> GSMQANQWQSVQNRTFTKWFNTKLSSRDLPSVFDLRKDLSDGILLIQLLEIIGDENLGRYNRNPRMRVHRLENVNKALEYIKSKGMPLTNIGPADIVDGNLKLILGLIWTLILRFTIADINEEGLTAKEGLLLWCQRKTANYHPEVDVQDFTRSWTNGLAFCALIHQHRPDLLDYNKLDKKNHRANMQLAFDIAQKSIGIPRLIEVEDVCDVDRPDERSIMTYVAEYFHAFSTLDK

α-actinin, a ubiquitous actin cross-linking and bundling protein, belongs to the spectrin superfamily. This group of proteins is characterized by a highly conserved N-terminal actin-binding domain, a central rod domain consisting of spectrin-like repeats and a calmodulin-like domain at the C-terminal (Blanchard, Ohanian & Critchley, 1989; Otey & Carpen, 2004; Sjöblom, Salmazo & Djinovic-Carugo, 2008). As α-actinin forms antiparallel homodimers, it can cross-link actin filaments, thereby contributing to the three-dimensional organization of the actin cytoskeleton. In S. pombe α-actinin appears to be expressed only during cell division and then localizes mainly to the contractile ring in an actin-dependent manner (Coffman et al., 2009; Wu, Bahler & Pringle, 2001).

The structure of S. pombe ABD consists of two calponin homology domains with similar folds, CH1 (residues 6–119) and CH2 (residues 120–234). Each domain consists of four long helices A1, C1, E1, G1 and A2, C2, E2 and G2 respectively. Indeed, the overall fold of S. pombe α-actinin ABD is very similar to other actin-binding domains. The structure was solved in the closed conformation where the interactions between the CH1 and CH2 domains are mainly caused by helices A1 and G1 (CH1 domain) and helix G2 and the coiled region between helices E2 and G2 (CH2 domain). The hydrogen bonding pattern between CH1 and CH2 is very much conserved when comparing S. pombe ABD with other ABDs. Further, there is a π-cation interaction between two residues from G1 and G2. In the S. pombe protein this interaction occurs between the conserved Trp107 and Arg216. In addition, there is a salt bridge present between helix A1 in CH1 and the loop between E2 and G2 in CH2 in the S. pombe protein; a strong bidentate hydrogen bond interaction between Arg12 and Asp206 (hydrogen bond distances: 2.9 and 3.1 Å, respectively). Taken together, the strength of the π-cation bond between Trp107 and Arg216 and the interaction between Arg12 and Asp206 indicate strong interactions between CH1 and CH2 and may favor a closed conformation of the actin-binding domain. Three metal ions are found in the crystal structure and they are modelled as zinc due to the high concentration of zinc in the crystallization conditions.> MSENSEIMKYVATTCPYCGVGCTLNLVVSNGKVVGVEPNQRSPINEGKLCPKGVTCWEHIHSPDRLTTPLIKKDGKFIEASWDEALDLVAKNLKVIYDKHGPKGLGFQTSCRTVNEDCYIFQKFARVGFKTNNVDNCARICHGPSVAGLSLSFGSGAATNGFEDALNADLILIWGSNAVEAHPLAGRRIAQAKKKGIQIIAVDPRYTMTARLADTYVRFNPSTHIALANSMMYWIIKE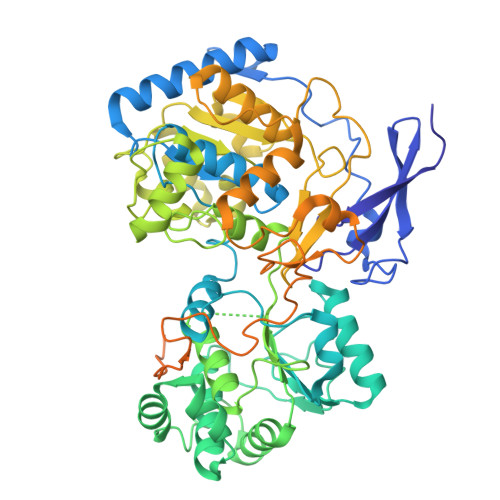GLEDKKFIQDRVNGFEDLKKTVENYADAEAIHGVPLDVVKDIAFRYAKAKNAVIIYCLGITELTTGTDNVRSMGNLALLTGNVGREGVGVNPLRGQNNVQGACDMGAYPNVYSGYQKCEVAENRAKMEKAWSVTNLPDWYGATLTEQINQCGDEIKGMYILGLNPVVTYPSSNHVKAQLEKLDFLVVQDIFFTETCQYADVILPGACFAEKDGTFTSGERRINRVRKAVNPPGQAKEDIHIISELAAKMGFKGFELPTAKDVWDDMRAVTPSMFGATYEKLERPEGICWPCPTEEHPGTPILHREKFATADGKGNLFGIDYRPPAEVADAEYPFTLMTGRLIFHYHSRTQTDRAADLHREVPESYAQINIEDARRLGIKNNEYIKLKSRRGETTTLARVTDEVAPGVVYMTMHFADGVNNLTNTVLDPMSKMPELKHCAISIEKVGGN4-PHENYL-1,2,5-OXADIAZOL-3-AMINE | C8 H7 N3 O | 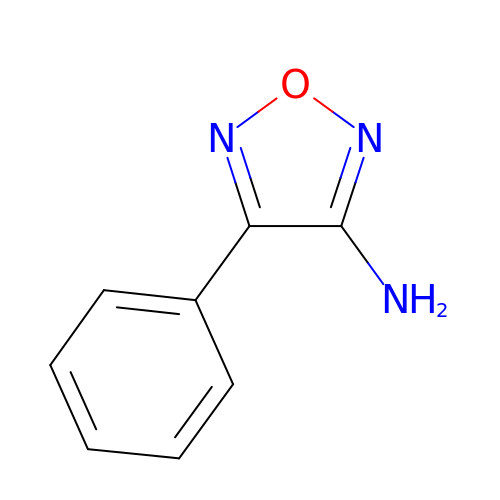APGIIVSHRRCAPU-UHFFFAOYSA-N1-(TERT-BUTYL)-3-(QUINOXALIN-6-YL)UREA | C13 H16 N4 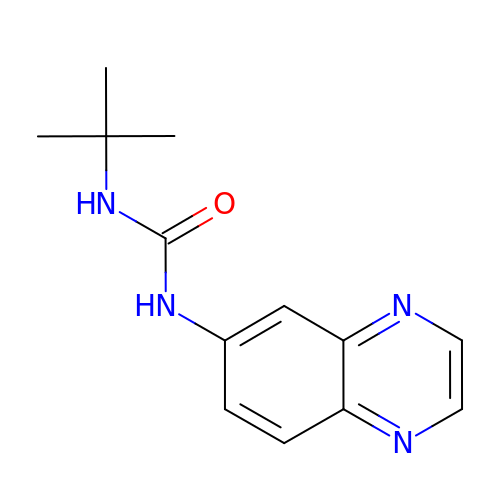O | LTTKIGSXIAQOSY-UHFFFAOYSA-N>[7x]MSMYTTAQLLAANEQKFKFDPLFLRLFFRESYPFTTEKVYLSQIPGLVNMALYVSPIVSGEVIRSRGGSTSEFTPGYVKPKHEVNPQMTLRRLPDEDPQNLADPAYRRRRIIMQNMRDEELAIAQVEEMQAVSAVLKGKYTMTGEAFDPVEVDMGRSEENNITQSGGTEWSKRDKSTYDPT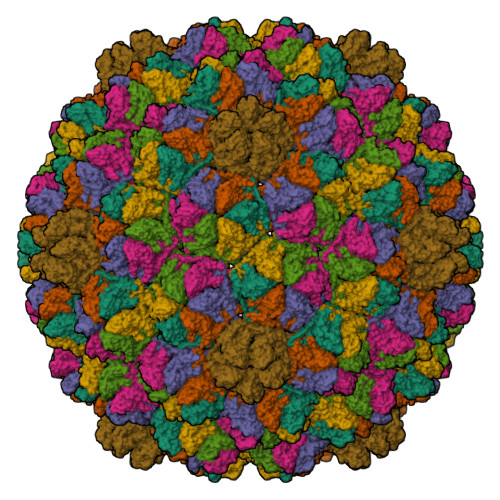DDIEAYALNASGVVNIIVFDPKGWALFRSFKAVKEKLDTRRGSNSELETAVKDLGKAVSYKGMYGDVAIVVYSGQYVENGVKKNFLPDNTMVLGNTQARGLRTYGCIQDADAQREGINASARYPKNWVTTGDPAREFTMIQSAPLMLLADPDEFVSVQLA R-BICALUTAMIDE | C18 H14 F4 N2 O4 S | 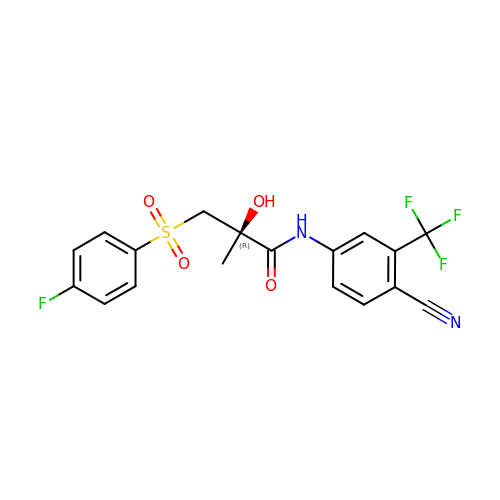LKJPYSCBVHEWIU-KRWDZBQOSA-N>MAPAMDSAQNGHQSRGSANVLAIGTANPPNVILQEDYPDFYFKVTNSEHLTDLKEKFKRICVKSKTRKRHFYLTEQILKENPGIATYGAGSLDSRQKILETEIPKLGKEAAMVAIQEWGQPVSKITHVVFATTSGFMMPGADYSITRLLGLNPNVRRVMIYNQGCFAGGTALRVAKDLAENNKGARVLVVCAENTAMTFHGPNENHLDVLVGQAMFSDGAAALIIGANPNLPEERPVYEMVAAHQTIVPESDGAIVAHFYEMGMSYFLKENVIPLFGNNIEACMEAAFKEYGISDWNSLFYSVHPGGRAIVDGIAEKLGLDEENLKATRHVLSEYGNMGSACVIFILDELRKKSKEEKKLTTGDGKEWGCLIGLGPGLTVETVVLRSVP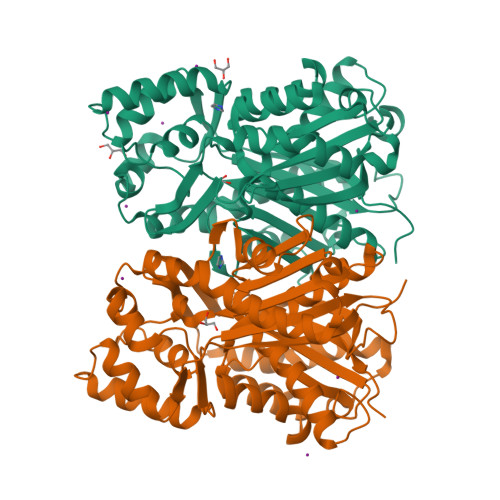IAAAALEHHHHHH[2x]> APTAPSIDMYGSNNLQFSKIELAMETTSGYNDMVKYHELAKIKVKFNQWSGTSGDTYNVYFDGVKVATGAITGSQTTASFEYGQGGL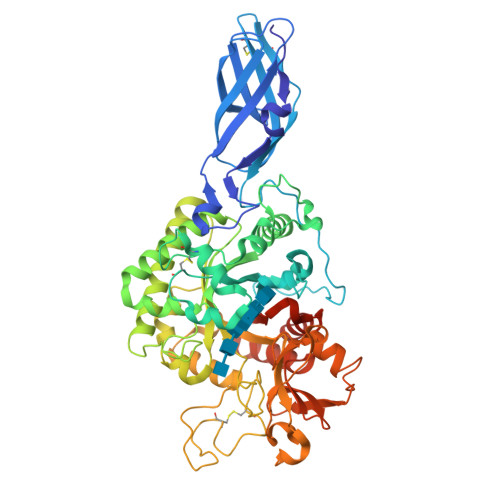YQMEIEACDATGCSKSAPVEITIADTDGSHLKPLTMNVDPNNKSYNTDPSIVMGTYFVEWGIYGRDYTVDNMPVDNLTHILYGFIPICGPNESVKSVGGNSFNALQTACRGVNDYEVVIHDPWAAYQKSFPQAGHEYSTPIKGNYAMLMALKQRNPDLKIIPSIGGWTLSDPFYDFVDKKNRDTFVASVKKFLKTWKFYDGVDIDWMFPGGGGAAADKGDPVNDGPAYIALMRELRVMLDELEAETGRTYELTSAIGVGYDKIEDVDYADAVQYMDYIFAMTYDFYGGWNNVPGHQTALYCGSFMRPGQCDGGGVDENGEPYKGPAYTADNGIQLLLAQGVPANKLVLGTAMYGRGWEGVTPDTLTDPNDPMTGTATGKLKGSTAQGVWEDGVIDYKGIKSFMLGANNTGINGFEYGYDAQAEAPWVWNRSTGELITFDDHRSVLAKGNYAKSLGLAGLFSWEIDADNGDILNAMHEGMAGGVVTPPNRRSHHHHHH2-[(2S)-1-azabicyclo[2.2.2]octan-2-yl]-6-(5-methyl-1H-pyrazol-4-yl)thieno[3,2-d]pyrimidin-4(3H)-one 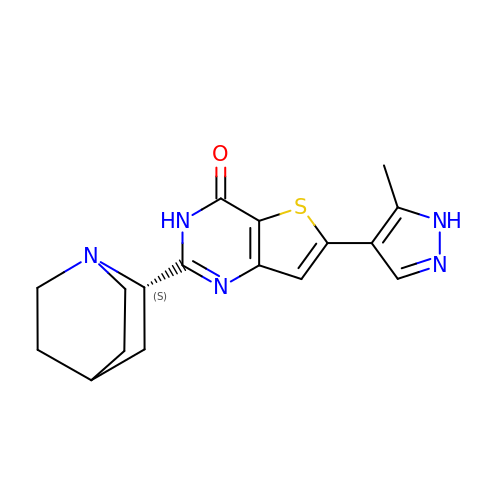| C17 H19 N5 O S | XGVXKJKTISMIOW-ZDUSSCGKSA-N> MELTPREKDKLLLFTAALVAERRLARGLKLNYPESVALISAFIMEGARDGKSVASLMEEGRHVLTREQVMEGVPEMIPDIQVEATFPDGSKLVTVHNPII;> MIPGEYHVKPGQIALNTGRATCRVVVENHGDRPIQVGSHYHFAEVNPALKFDRQQAAGYRLNIPAGTAVRFEPGQKREVELVAFAGHRAVFGFRGEVMGPLEVNDE;> MSNISRQAYADMFGPTVGDKVRLADTELWIEVEDDLTTYGEEVKFGGGKVIRDGMGQGQMLAADCVDLVLTNALIVDHWGIVK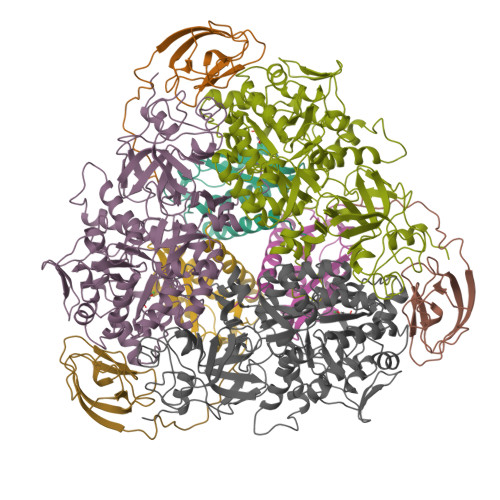ADIGVKDGRIFAIGKAGNPDIQPNVTIPIGAATEVIAAEGKIVTAGGIDTHIHWICPQQAEEALVSGVTTMVGGGTGPAAGTHATTCTPGPWYISRMLQAADSLPVNIGLLGKGNVSQPDALREQVAAGVIGLKIHEDWGATPAAIDCALTVADEMDIQVALHSDTLNESGFVEDTLAAIGGRTIHTFHTEGAGGGHAPDIITACAHPNILPSSTNPTLPYTLNTIDEHLDMLMVSHHLDPDIAEDVAFAESRIRRETIAAEDVLHDLGAFSLTSSDSQAMGRVGEVILRTWQVAHRMKVQRGALAEETGDNDNFRVKRYIAKYTINPALTHGIAHEVGSIEVGKLADLVVWSPAFFGVKPATVIKGGMIAIAPMGDINASIPTPQPVHYRPMFGALGSARHHCRLTFLSQAAAANGVAERLNLRSAIAVVKGCRTVQKADMVHNSLQPNITVDAQTYEVRVDGELITSEPADVLPMAQRYFLF>[2x]MGFKCGI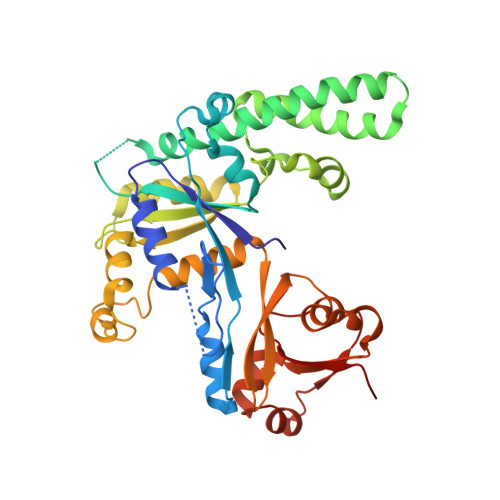VGLPNVGKSTLFNALTKAGIEAANYPFCTIEPNTGVVPMPDPRLDALAEIVKPERILPTTMEFVDIAGLVAGASKGEGLGNKFLANIRETDAIGHVVRCFENDDIVHVAGKIDPLDDIDTINTELALADLDSCERAIQRLQKRAKGGDKEAKFELSVMEKILPVLENAGMIRSVGLDKEELQAIKSYNFLTLKPTMYIANVNEDGFENNPYLDRVREIAAKEGAVVVPVCAAIESEIAELDDEEKVEFLQDLGIEEPGLNRVIRAGYALLNLQTYFTAGVKEVRAWTVSVGATAPKAAAVIHTDFEKGFIRAEVIAYEDFIQFNGENGAKEAGKWRLEGKDYIVQDGDVMHFRFNV>[3x]GAGAGSKRIQLEPL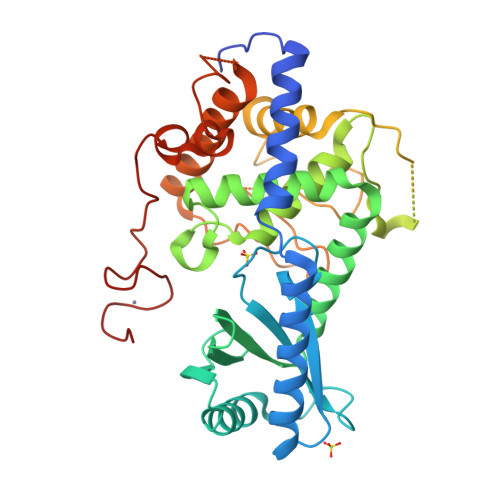PPLTPKFLNILDQVCIQCYKDFSPTIIEDQAREHIRQNLESFIRQDFPGTKLSLFGSSKNGFGFKQSDLAVCMTINGLETAEGLDCVRTIEELARVLRKHSGLRNILPITTAKVPIVKFFHLRSGLEVDISLYNTLALHNTRLLSAYSAIDPRVKYLCYTMKVFTKMCDIGDASRGSLSSYAYTLMVLYFLQQRNPPVIPVLQEIYKGEKKPEIFVDGWNIYFFDQIDELPTYWSECGKNTESVGQLWLGLLRFYTEEFDFKEHVISIRRKSLLTTFKKQWTSKYIVIEDPFDLNHNLGAGLSRKMTNFIMKAFINGRRVFGIPVKGFPKDYPSKMEYFFDPDVLTEGELAPNDRCCRICGKIGHFMKDCPMRRK> GRKRRQTS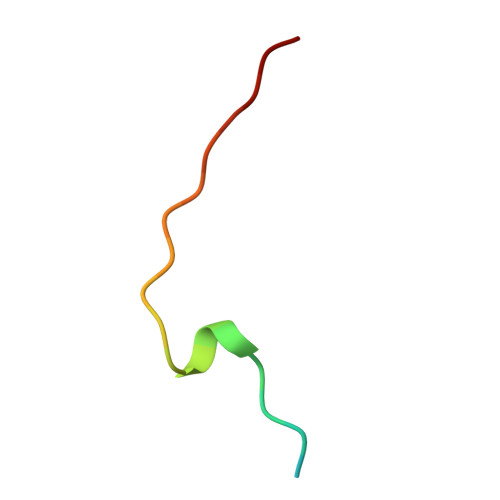MTDFYHSKRRLIFS> DQSDPEDVGKMTTENNIVVDKSDLIPKVLTLNV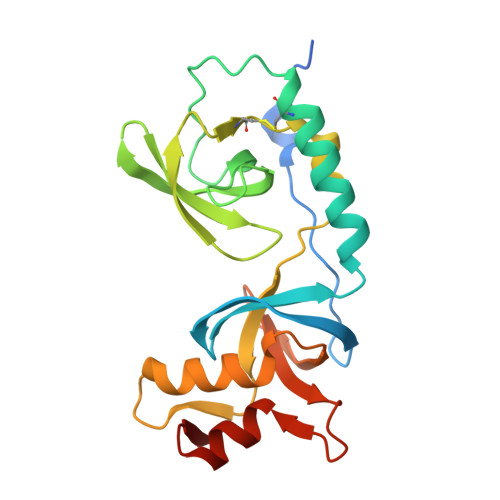GDEFCGVVAHIQTPEDFFCQQLQSGRKLAELQASLSKYCDQLPPRSDFYPAIGDICCAQFSEDDQWYRASVLAYASEESVLVGYVDYGNFEILSLMRLCPIIPKLLELPMQAIKCVLAGVKPSLGIWTPEAICLMKKLVQNKIITVKVVDKLENSSLVELIDKSETPHVSVSKVLLDAGFAVGEQSM> MALFGTKDTTTAHSDYEIILEGGSSSWGQIKGRAKVNVPAALPLLPADCNIKIEAKPLDAQKGVVRFTSQIESIVDSTKNKLVVEVDIANETKDRRIAVGEGEVSVGDFSHKFSFEGSVVNMYYYRSDAVRRNVPNPVYMQGRQFHDIMMKVPLDNKDLIETWEGFQQSISGGGVNFGDWIREFWFIGPAYT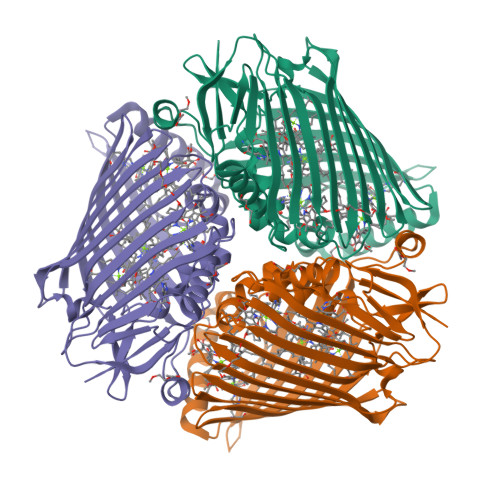AINEGGQRISPIQVNNFGVESGEKGPVGVSRWKFSHAGSGIVDSISRWAELFPVEQLNKPASIEGGFRSDSQGIEVKVDGNLPGVSRDAGGGLRRILNHPLIPLVHHGMVGKFNDFTVDTQLKVVLPKGYKIRYAAPQFRSQNLEEYRWSGGAYARWVEHVCKGGTGQFEVLYAQ>GSMSLKPFTYPFPETRFLHAGPNVYKFKIRYGKSIRGEEIENKEVITQELEDS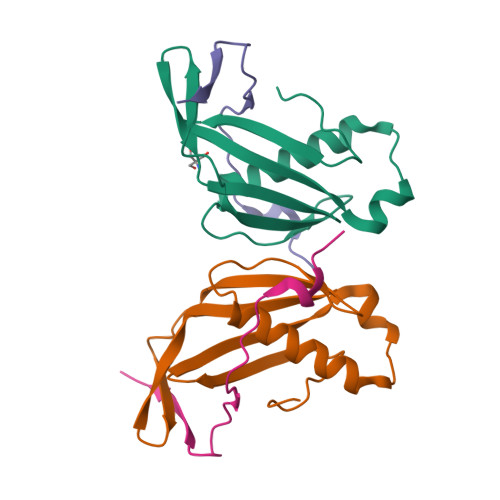VRVVLGNLDNLQPFATEHFIVFPYKSKWERVSHLKFKHGEIILIPYPFVFTLYVE[2x];>GSMPVNNMVTGYISIDAMKKFLGELHDFIPGTSGYLAYHVQNE[2x]> MYRLGSQGRSIQSQLQNGDSSSGRPLQLQGTGMREAQRIPQQLDYLLAEIISPNEDTNVIGYLAYYYPKLKNEQNVALLTDFFLRCPTYFSHSNVVSLRNNYPVMEAFNYIMTTKFKVSQPTVPFYRFYAAVLASLLNCEKTDPSHHWKLIPILTGVLLSIKGRDDVELYPDHSRSIKGSDTAVAQLLQRCLLRFYQSGDARSYDLNALVIISMSCALDYVEDDTIKKILYCFNYTRAIIDLIYYSPYGLNDSDIPLLSDSSVNSQSFDQLLNNNPALKHLNRLSFLFERTVKLNDGSIQSNLNDIDISLNKMQSFSEKLSKKISVLDDDSSKGVGQLLRQCLYASIIIHQAILTTFFQLDNADYTKYFLPSFSRKILSILFNLFFIVDRIGTGGFQPYNFVYLTCLQGIIQYDMKTAESLVKTFTTGINYSSLKDSEVARAKLLFTLNLMEQIVNICSDDLRLELIVPLVEDLVNNKNACVDIHNHVFK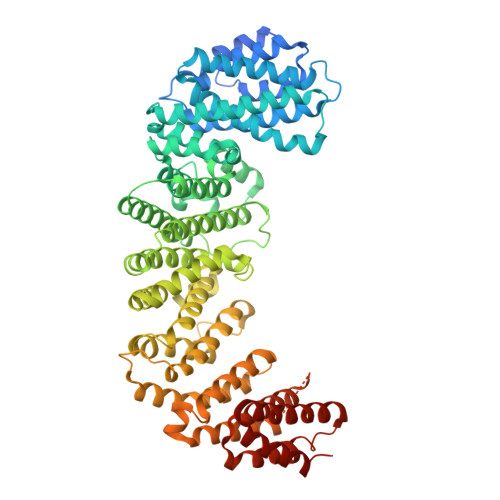SIFESAHSVILKFFTVVDSSVKNVDYETNVTLVSEKIIPYLTLVIDQFPEFLSINQLDIAIETISRTVFPDSPIYSYDKNISSMFLNVLFNKCLTVDNDELVELPAIEAVVAPKNDEENNTSDAQDGGPKELQSLNDLKSRRSALISALISVFPLIPVKDYTKWLSIAFYDLIVATPERTERAFLQERLWDCVVGTNKYDPQKGNLGIMWWYENVNAQSTAKL>[2x]MGEKALPVVYKRYICSFADCGAAYNKNWKLQAHLCKHTGEKPF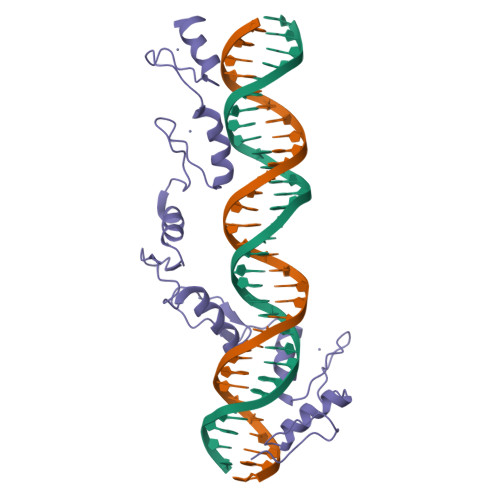PCKEEGCEKGFTSLHHLTRHSLTHTGEKNFTCDSDGCDLRFTTKANMKKHFNRFHNIKICVYVCHFENCGKAFKKHNQLKVHQFSHTQQLPYECPHEGCDKRFSLPSRLKRHEKVHAGYPCKKDDSCSFVGKTWTLYLKHVAECHQD> MVRGRVPQIQARQINIFGIVQGVGFRPFVFNIAQKYNLKGIVYNNSSGLYIEVEGEEKDIEAFIREIKENPPSLSVIDEIQVREVEVKEYKDFKIVGSKEDGGFVPVSPDMGVCEDCLRELKDPK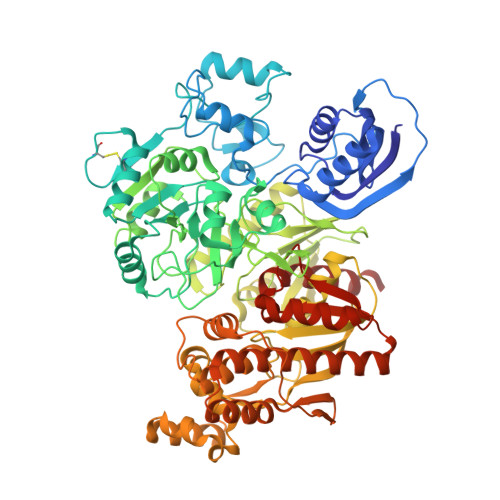DRRYRYPFINCTNCGPRFSIIEDIPYDRAKTSMKVFPMCEKCSREYHDPHDRRFHAQPVACFDCGPSLSFVGEGCFDDEIKCVAKALKEGKIVAIKGIGGFHLAVNALDDEAVATLRRRKKRYGKPFAVMMRDVEEVKKYCIVSPEEERLLLSQRRPIVLLKKKGEKLAKGIADDLDTLGVMLPYAPIHYLLMEEIDFPIVMTSGNVSEEPICKDNEEALEKLKDIADVFLLNNRDIVNRIDDSVTSFNAGAERIIRRARGYAPQPILLKKEVKASILAVGGFYKNTFCMTKGHYAFISHHIGDLDNEKAFNYYIEQIERYKKLFRVDPEVVAHDMHKGYLSTQYAKSLDLPKIEVQHHHAHIASCMAEHNLDEKVIGIAYDGTGYGTDGNVWGAEILVCDLKSFERIAHLKYKPLPGNELAIKKIYRTALGFIFDNISFYKNFVEQVDSRELDIILKQIDRKINTAYVSSMGRFFDAVAALIGVRKEVLFEGQAAMELESLMAESEEYYEYEILKEDRYVIDPELILRQIYEDYMKGFEKSYISAKFHNTVVNFTYDLANLIRKETGINKVVLSGGSFQNRYLLRRLIEKLSLSGFEVYSNSKVPCNDGGISLGQAVIANKILEGSAWSHPQFEK>[2x]SGLTPIHVAAFMGHLNIVLLLLQNGASPDVTNIRGETALHMAARAGQVEVVRCLLRNGALVDARAR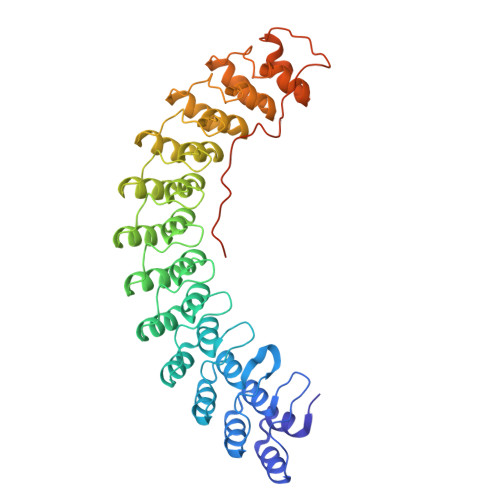EEQTPLHIASRLGKTEIVQLLLQHMAHPDAATTNGYTPLHISAREGQVDVASVLLEAGAAHSLATKKGFTPLHVAAKYGSLDVAKLLLQRRAAADSAGKNGLTPLHVAAHYDNQKVALLLLEKGASPHATAKNGYTPLHIAAKKNQMQIASTLLNYGAETNIVTKQGVTPLHLASQEGHTDMVTLLLDKGANIHMSTKSGLTSLHLAAQEDKVNVADILTKHGADQDAHTKLGYTPLIVACHYGNVKMVNFLLKQGANVNAKTKNGYTPLHQAAQQGHTHIINVLLQHGAKPNATTANGNTALAIAKRLGYISVVDTLKVVTEEVTTTTTTITEKHKLNVPETMTEVLDVSDEEGDDTMTGDGGEYLRPEDLKELGDD Organic cation transporters (OCTs) facilitate the translocation of catecholamines, drugs and xenobiotics across the plasma membrane in various tissues throughout the human body. Organic cation transporter 3 (OCT3, SLC22A3) was identified as a corticosterone-sensitive catecholamine transporter in 1998 and belongs to the SLC22 family of the major facilitator superfamily (MFS) of transporters. OCT3 plays a key role in low-affinity, high-capacity uptake of monoamines in most tissues including heart, brain and liver. The substrate binding site is located in the center of the transporter between the two domains, halfway through the membrane.

We purified and reconstituted OCT3 into nanodiscs (MSP1D1 filled with brain polar lipids) and subjected the sample to extensive cryo-EM data collection and image processing. We obtained a 3D reconstruction of OCT3 (apo-state) at 3.2 Å resolution and completed the model by combining the experimentally determined structure with an in silico model generated by AlphaFold (detailed in Materials and Methods). The structure features a prominent, partially resolved density of the extended extracellular loop 1 or ectodomain (ECD), which is adjacent to the outward-open translocation pathway. The structure of OCT3 features various negatively charged residues lining the substrate translocation pathway: D155, E232, D382, E390, E451, E459 and D478. The outward-open state of the lipid-reconstituted OCT3 is surrounded by several lipid densities. The protein structure features a V-shaped lateral opening at the interface between the two halves of the protein (“V-site”). Several conserved lipid densities are present at this site, indicating the margins of the lipid bilayer. We presently cannot unambiguously assign the identity of the lipids in this region (brain polar lipids, which include cholesterol and phospholipids, were used for nanodisc reconstitution). This V-site may serve as an access pathway for hydrophobic molecules that diffuse into the OCT3 translocation pathway. In apo OCT3, this network is very dynamic, as R212 cannot establish all interactions simultaneously. OCT3 shows an obvious access path to the substrate binding site that is wide open to the extracellular side.

> MPSFDEALQRVGEFGRFQRRVFLLLCLTGVTFAFLFVGVVFLGTQPDHYWCRGPSAAALAERCGWSPEEEWNRTAPASRGPEPPERRGRCQRYLLEAANDSASATSALSCADPLAAFPNRSAPLVPCRGGWRYAQAHSTIVSEFDLVCVNAWMLDLTQAILNLGFLTGAFTLGYAADRYGRIVIYLLSCLGVGVTGVVVAFAPNFPVFVIFRFLQGVFGKGTWMTCYVIVTEIVGSKQRRIVGIVIQMFFTLGIIILPGIAYFIPNWQGIQLAITLPSFLFLLYYWVVPESPRWLITRKKGDKALQILRRIAKCNGKYLSSNYSEITVTDEEVSNPSFLDLVRTPQMRKCTLILMFAWFTSAVVYQGLVMRLGIIGGNLYIDFFISGVVELPGALLILLTIERLGRRLPFAASNIVAGVACLVTAFLPEGIAWLRTTVATLGRLGITMAFEIVYLVNSELYPTTLRNFGVSLCSGLCDFGGIIAPFLLFRLAAVWLELPLIIFGILASICGGLVMLLPETKGIALPETVDDVEKLGSPHSCKCGRNKKTPVSRSHL> MIVLFVD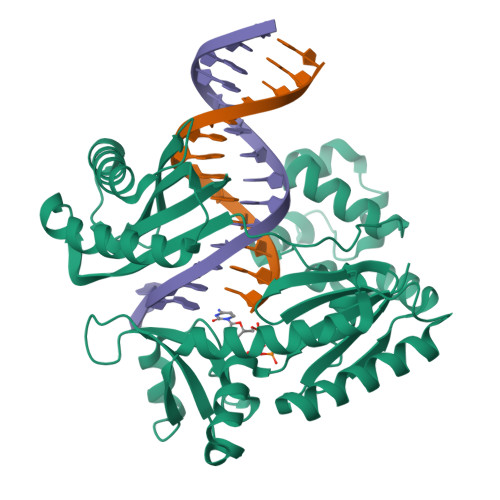FDYFYAQVEEVLNPSLKGKPVVVCVFSGRFEDSGAVATANYEARKFGVKAGIPIVEAKKILPNAVYLPMRKEVYQQVSSRIMNLLREYSEKIEIASIDEAYLDISDKVRDYREAYNLGLEIKNKILEKEKITVTVGISKNKVFAKIAADMAKPNGIKVIDDEEVKRLIRELDIADVPGIGNITAEKLKKLGINKLVDTLSIEFDKLKGMIGEAKAKYLISLARDEYNEPIRTRVRKSIGRIVTMKRNSRNLEEIKPYLFRAIEESYYKLDKRIPKAIHVVAVTEDLDIVSRGRTFPHGISKETAYSESVKLLQKILEEDERKIRRIGVRFSKFILEHHHHHH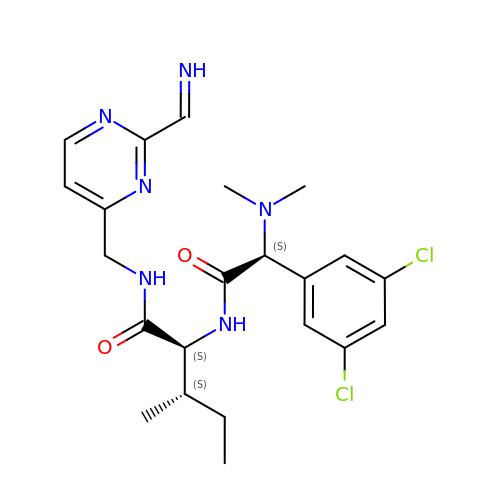(2~{S},3~{S})-2-[[(2~{S})-2-[3,5-bis(chloranyl)phenyl]-2-(dimethylamino)ethanoyl]amino]-~{N}-[[2-(iminomethyl)pyrimidin-4-yl]methyl]-3-methyl-pentanamide | C22 H28 Cl2 N6 O2 | XBUAFLLXSYLZPV-BFFNQEOMSA-N> MVTEMSHAESIKRVVDQKLSSHEGFESHMFKIGSYNEAVGESSPFALPYDDSTMALLILSTPDMFDVAFRKWVVQKTMDFGSFDEVCEMVSSPIQSFLEDRLEIMSEKLRKVEENFEILHDYSMTPQRRPKILMQTCGHVAGAAFYYQPCHFQEDGVTWPPAGRMGPNLKFIGLSLHPIYGGHFAFRSVLIFPNVKIPEFCEKEPRPILTASEDVRTALEKFNYNWKDSGFRDFGNPTRRYSTTQMEFFGRPVAERWEVLRP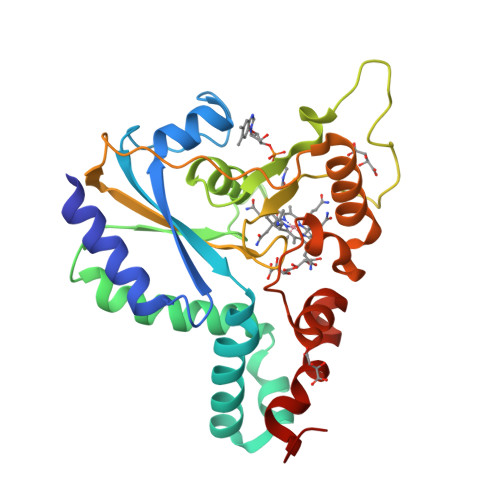WVENLYFQ> GLVKNEDVTAESSLTMTSVALTEKQSEEKRKKLDALSAEIGQFLAQAQGLPNSNEAITKASLAKNEIVEALKGEVSDLAPILQKATEARNSIANAVLRANSGLRDSRNGQALTKASNTASFRAARDTEKPELQKITVTGGAVLEGQKFKIYREENFSATIEFTDNSGRIEHAKFVPTAVPAAYPATSTVVSFTTSNGQSISMIVPTNKLAKDGNATASNPFTVSITGSVGKNQAVNSLWTRYVFTYDQEGNFSGNTTDVGLVKDLTANPAAIQFEVHAQSEKYEPAINAEVNRNFTLTANSGTVSVGEASQYITNATGTPELPTTGITKGTRTTYTWKSGTNTNLSAGRHTLTAVVTYPDGSTDEIDVSFTVRPQTPRIEERFLNEKGGLTNQAITVDGVTPGGTVTLTIAGETFTKQATGSSTSVTFTANELKKVYDRNGGRLPSGPVTASTTVNG

The long-wavelength beamline I23 at Diamond Light Source overcomes these limitations and extends the accessible wavelength range to λ = 5.9 Å. In this study, we report the determination of diverse protein structures by experimental phasing techniques carried out at long wavelengths on beamline I23 at Diamond Light Source using S, Ca, K, Cl, V, I, Cd, and P as anomalous scatterers. Native-SAD uses light atoms naturally occurring in proteins or bound to proteins. We demonstrate that long-wavelength native-SAD has become a very compelling technique, where a low multiplicity dataset from a single crystal can be sufficient for successful structure determination, making it a general vehicle of choice for experimental phasing.

Calcium is used less often because its K-edge is located at a longer wavelength (λ = 3.07 Å), typically not accessible at standard MX beamlines. A domain of the accessory Sec-dependent serine-rich glycoprotein adhesin from Streptococcus oralis (Fap1) was solved by Ca-SAD on beamline I23 from two calcium ions and 1080° of data to a resolution of 2 Å. Compared to sulfur, the calcium anomalous signal is stronger and more efficient for phasing.>EPLDIEAYAALYKGRTKIMRLLFIANHCGGNHALQFDALRMAYDEIKKGENTQLFREVVNKIGNRLGEKYGMDLAWCEAVDRRAEQKKVKLENELSSYRTNLIKESIRMGYNDFGDFYYACGMLGDAFKNYIRTRDYCTTTKHIIHMCMNAILVSIEMGQFTHVTSYVNKAEQNPETLEPMVNAKLRCASGLAHLELKKYKLAARKFLDVNPELGN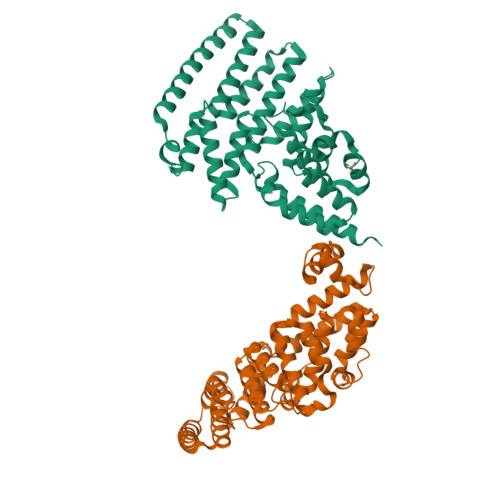SYNEVIAPQDIATYGGLCALASFDRSELKQKVIDNINFRNFLELVPDVRELINDFYSSRYASCLEYLASLKSNLLLDIHLHDHVDTLYDQIRKKALIQYTLPFVSVDLSRMADAFKTSVSGLEKELEALITD[4x]>[8x]SNAEGLRRHSVMLDCKLWKDDPIYFFKTLPPYISKYAQRADDASIQAQIDVFGKDDVGAMPGALGPRGNFAAVTFAESFPDRVAMLAYLNEVLSFYECFEKQMTEMLDATLYANPVPKDPKYDNPVWQANYKNTMTKWPKILENLDPK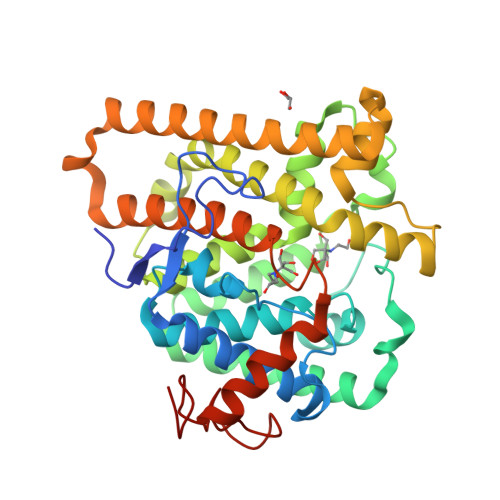LGPKCVKSLVALVEGTDMEPKMAHYKTMKEYALDRTNYIAWPVACDNAEFGSQLNLTQDQLDSVRDIFLPLWTHSCYVYDYYHYDKEAEIHSTYGKGRSMINSIPLLNRLKGLSVEEAKAWLKQRCFELEKEYLQRKEDYFSENPVEAVPVDLRRWFLSQEDLATGFAIWCATTYHNHPPFGEGYAAPYEKRRKEGALWFEKVTESDQLMTGGFEVRYAN>SNAMRVISGEYGGRRLKAL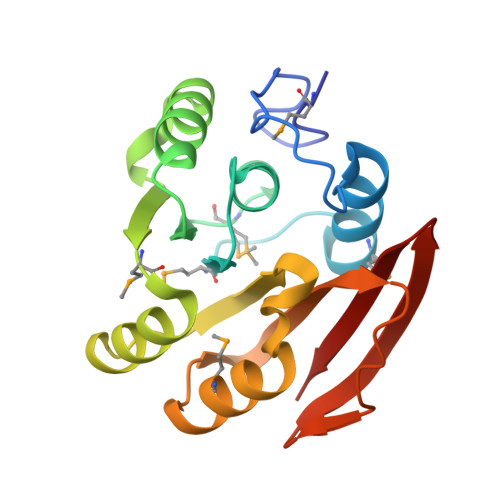DGDNTRPTTDKVKESIFNMIGPYFDGGMALDLYSGSGGLAIEAVSRGMDKSICIEKNFAALKVIKENIAITKEPEKFEVRKMDANRALEQFYEEKLQFDLVLLDPPYAKQEIVSQLEKMLERQLLTNEAVIVCETDKTVKLPETIGTLKKTRETVYGITQVTIYRQEA[2x]> GPGGSGGVTEEQVHHIVKQALQ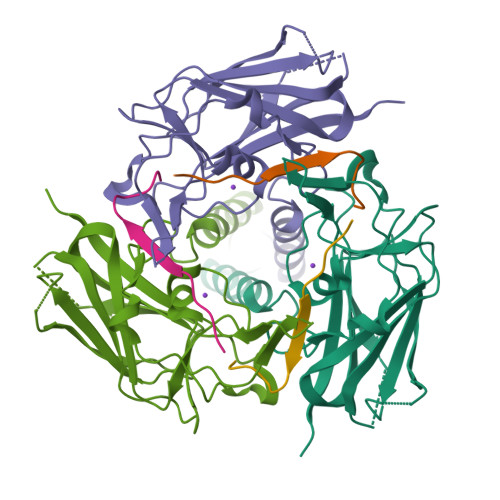RYSEDRIGLADYALESGGASVISTRCSETYETKTALLSLFGIPLWYHSQSPRVILQPDVHPGNCWAFQGPQGFAVVRLSARIRPTAVTLEHVPKALSPNSTISSAPKDFAIFGFDEDLQQEGTLLGKFTYDQDGEPIQTFHFQAPTMGTYQVVELRILTNWGHPEYTCIYRFRVHGEPAH;> GPGGSGGPSPPPTWPHLQLCYLQPPPV> HAQPPPQPRKKRPEDFKFGKILGEGSFSTVVLARELATSREYAIKILEKRHIIKENKVPYVTRERDVMSRLDHPFFVKLYFTFQDDEKLYFGLSYAKNGELLKYIRKIGSFDETCTRFYTAEIVSALEYLHGKGIIHRDLKPENILLNEDMHIQITDFGTAKVLSPESKQARANSFVGTAQYVSPELLTEKSACKSSDLWALGCIIYQLVAGLPPFRAGNEYLIFQKIIKLEYDFPEKFFPKARDLVEKLLVLDATKRLGCEEMEGYGPLKAHPFF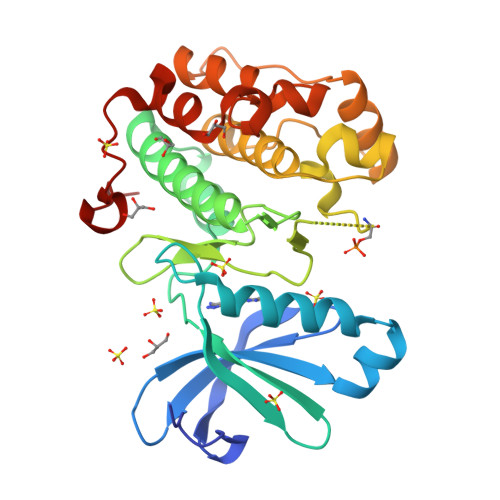ESVTWENLHQQTPPKL> HSSLTERHKILHRLL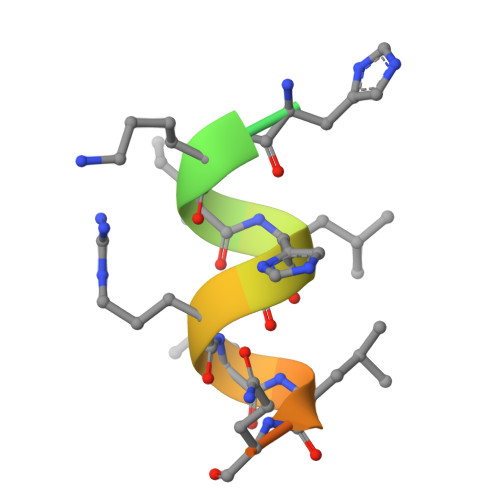QEGSPS4-METHYL-HISTIDINE | C7 H11 N3 O2 | 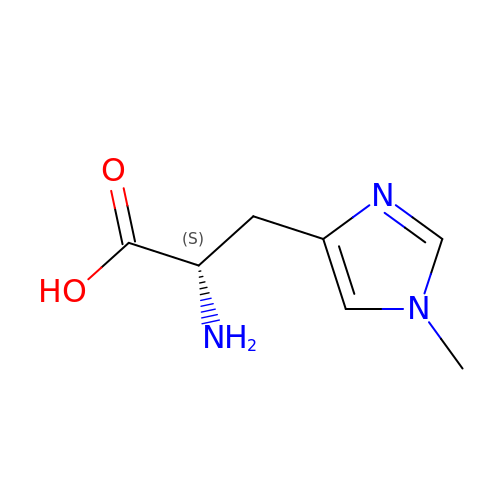BRMWTNUJHUMWMS-LURJTMIESA-N> SARSCTIHKEDLQDGLPVLIPKEDSLLYAGSVRTLQPPDIYSIVIEGERG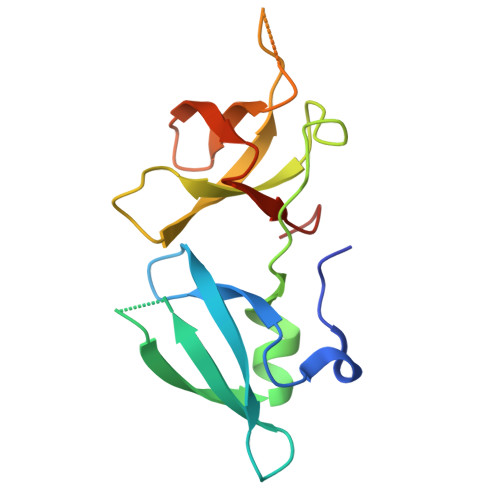NRQRIYSLEQLLQEAVLDVQPQSSRYLPPGTRVCAYWSQKSRCLYPGNVVRGASSDEEDLDSVLVEFDDGDTGHIAVSNIRLLPPDFKIQC>[14x]MHRTYSLRNSRAPTASQLQNPPPPPSTTKGRFFGKGGLAYSFRRSAAGAFGPELSRKLSQLVKIEKNVLRSMELTANERRDAAKQLSIWGLENDDDVSDITDKLGVLIYEVSELDDQFIDRYDQYRLTLKSIRDIEGSVQPSRDRKDKITDKIAYLKYKDPQSPKIEVLEQELVRAEAESLVAEAQLS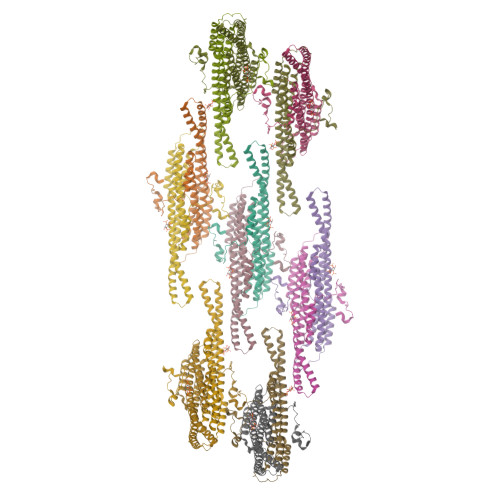NITRSKLRAAFNYQFDSIIEHSEKIALIAGYGKALLELLDDSPVTPGETRPAYDGYEASKQIIIDAESALNEWTLDSAQVKPTLSFKQDYEDFEPEEGEEEEEEDGQGRWSEDEQEDGQIEEPEQEEEGAVEEHEQVGHQQSESLPQQTTA>[16x]WIENIPLAEEEHNKWHQDAVSLHLEFGIPRTAAEDIVQQCDVCQENKMPSTLRGSNKRGIDHWQVDYTHYEDKIILVWVETNSGLIYAERVKGETGQEFRVQTMKWYAMFAPKSLQSDNGPAFVAESTQLLMKYLGIEHTTGIPWNPQSQALVERTHQTLKNTLEKLIPMFNAFESALAGTLITLNIKRKGGLGTSPMDIFIFNKEQQRIQQQSKSKQEKIRFCYYRTRKRGHPGEWQGPTQVLWGGDGAIVVKDRGTDRYLVIANKDVKFIPPPKEIQKE

A multimer of retroviral integrase (IN) synapses viral DNA ends within a stable intasome nucleoprotein complex for integration into a host cell genome. Reconstitution of the intasome from the maedi-visna virus (MVV), an ovine lentivirus, revealed a large assembly containing sixteen IN subunits. Retroviral integrase (IN), the enzyme responsible for this process, catalyzes two consecutive reactions: (i) 3′-processing, during which IN hydrolyses 2–3 nucleotides at the vDNA ends to liberate 3′-hydroxyls attached to invariant CA dinucleotides, and (ii) strand transfer, wherein IN utilizes the 3′-hydroxyls to cleave the chromosomal DNA, simultaneously joining the 3′ vDNA ends to target DNA (tDNA) strands. The amino-terminal domain (NTD) consists of a compact three-helical bundle stabilized by coordination of a Zn2+ ion; the catalytic core domain (CCD) features the RNaseH fold and harbors the invariant D,D-35-E catalytic triad; and the carboxy-terminal domain (CTD) adopts an SH3-like beta-barrel structure (reviewed in Jaskolski et al.).

Here, we describe high-resolution structures of the MVV intasome in two functional states: (i) prior to engagement of tDNA and (ii) following strand transfer. We collected single-particle cryo-EM data on the MVV intasome assembled in the form of the CSC and purified under conditions used in our previous study. The reconstruction was refined to an overall resolution of 3.4 Å. In agreement with the previously reported MVV CSC structure, which was refined to ~5 Å resolution, the present reconstruction lacked features consistent with LEDGF/p75. The CSC and STC structures recapitulated the MVV intasome architecture harboring sixteen IN subunits in a tetramer-of-tetramers arrangement. The CIC is formed from a pair of CCD dimers provided by IN tetramers I and II, plus a pair of synaptic CTDs derived from IN tetramers III and IV. Comparison of the CSC and STC structures confirmed that the intasome does not undergo extensive conformational changes upon tDNA binding and strand transfer. The CTDs from eight IN subunits form a pair of C2 symmetry-equivalent tetrads stabilizing the hexadecameric assembly via intra- and inter-tetramer CTD-CTD interactions as well as via contacts with vDNA. Importantly, the lentiviral intasomes share two unique features: intra-tetramer CTD-CTD contacts and an α-helical configuration of the CCD-CTD linkers. Using site-directed mutagenesis, we demonstrate that the hexadecameric assembly is essential for MVV IN strand transfer activity and virus infectivity.{4-[2-(2-hydroxyethoxy)phenyl]piperazin-1-yl}[(2R,3S)-2-propyl-3-[4-(trifluoromethyl)phenoxy]-1-{[4-(trifluoromethyl)pyridin-3-yl]carbonyl}piperidin-3-yl]methanone 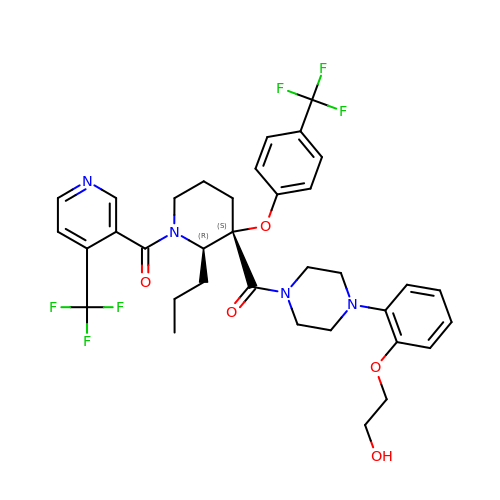| C35 H38 F6 N4 O5 | YHNPRKVZFODOHZ-NDKRRWIDSA-N>MNHKVHMMSKPVLYYDDISPPVRGVLLTVAALGIKDQVELKLVRLFEREHLLEDFVKLNPLHAVPVLKHDDLVLTDSHAIIMYLCDIFGQDGDFSLKDPKQRARVHNRLCFNNAVLFQRESIVMRGLINRSIVTLEDHHLKPVQEAYDCL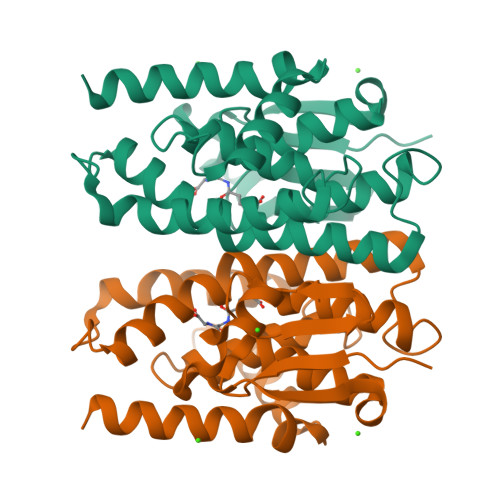EVYLTNSKFVACDQLTVADFPIVACMSTVGMVCPLSTSRWPKTAAWFETMKQLPYYQQANQVGVDKLKERLHAVMKK[4x]>[4x]MGFKEYPAGEPVTMNEMELAAVYLQPIDMEPRGMGLPAAKADVHLEADIHAVEGNKNGFGAGEWIPYLTISYTLVNNDTG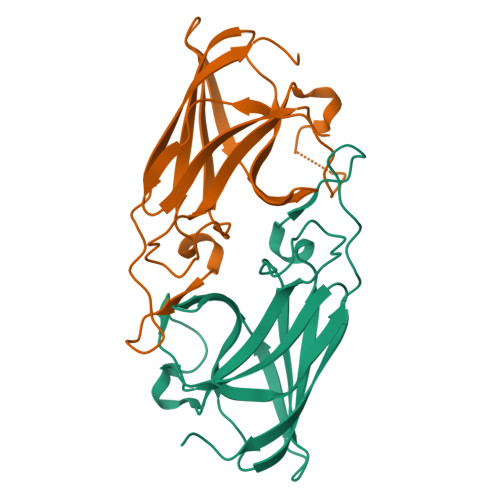EKQEGTFMPMVASDGPHYGANIKMMGVGNYKVTYHIEPPSKAGMHRHTDSETGVGRWWKPFDVSYEFKYVGLNSSGLVPR> ISGGDAIYSSTGRCSLGFNVRSGSTYYFLTAGHCTDGATTWWANSARTTVLGTTSGSSFPNNDYGIVRYTNTTIPKDGTVGGQDITSAANATVGMAVTRRGSTTGTHSGSVTALNATVNYGGGDVVYGMIRTNVCAEPGDSGGPLYSGTRAIGLTSGGSGNCSSGGTTFFQPVTEALVAYGVSVY;> VDCSEYPKPACTXEYRPLCGSDNKTYGNKCNFCNAVVESNGTL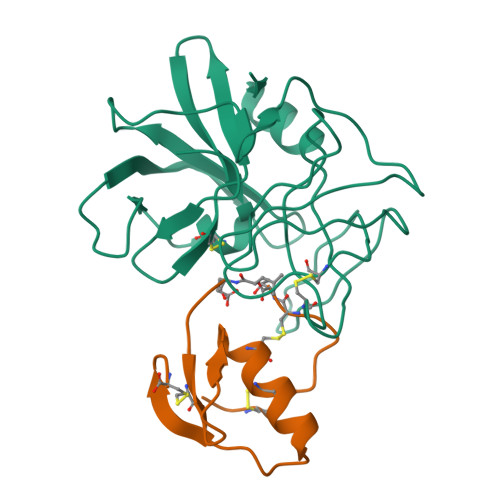TLSHFGKC>MKQLTILGSTGSIGCSTLDVVRHNPEHFRVVALVAGKNVTRMVEQCLEFSPRYAVMDDEASAKLLKTMLQQQGSRTEVLSGQQAACDMAALEDVDQVMAAIVGAAGLLPTLAAIRAGKTILLANKESLVTCGRLFMDAVKQSKAQLLPVDSEHNAIFQSLPQPIQHNLGYADLEQNGVVSILLTGSGGPFRETPLRDLATMTPDQACRHPNWSMGRKISVDSATMMNKGLEYIEARWLFNASASQMEVLIHPQSVIHSMVRYQDGSVLAQLGEPDMRTPIAHTMAWPNRVNSGVKPLDFCKLSALTFAAPDYDRYPCLKLAMEAFEQGQAATTALNAANEITVAAFLAQQIRFTDIAALNLSVL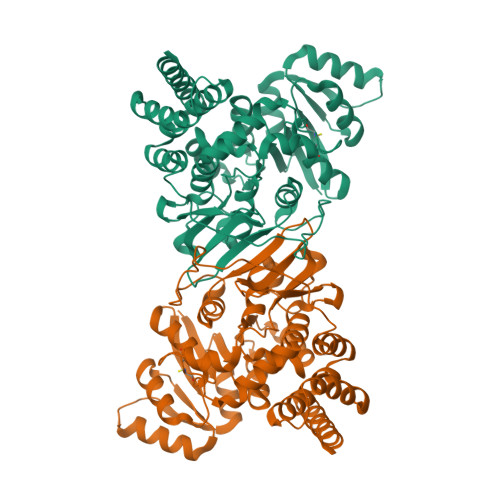EKMDMREPQCVDDVLSVDANAREVARKEVMRLAS[3x]>[6x]DADPTFDFIGYLET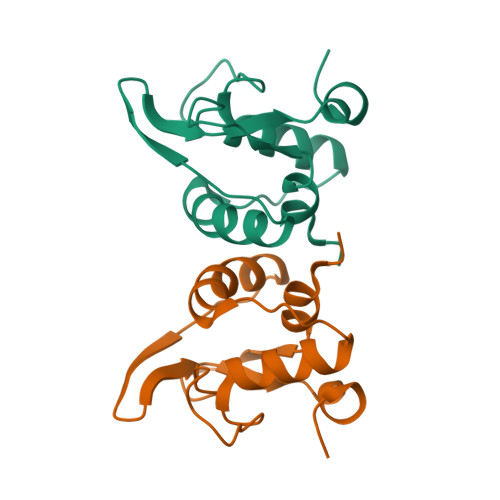LPQTSGMYMGNASIIPRNYRKYLYHAYLAYMEANGYRNVLSLKMFGLGLPVMLKEYGLNYEKRHTKQGIQTNLTLKEESYGDWLPK3-azanyl-2-[[(3~{S})-2,5-bis(oxidanylidene)pyrrolidin-3-yl]carbamoyl]benzoic acid | C12 H11 N3 O5 | 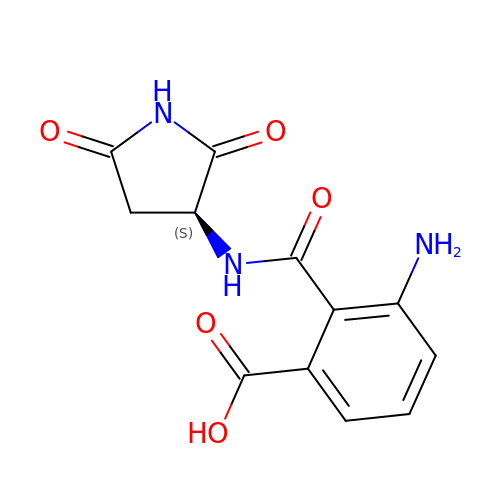OHXATMBWWVLISO-ZETCQYMHSA-N N-[(3aR,6aS)-hexahydrocyclopenta[c]pyrrol-2(1H)-ylcarbamoyl]-4-methylbenzenesulfonamide 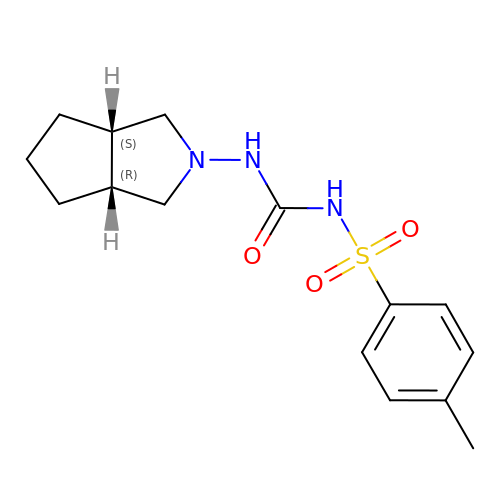| C15 H21 N3 O3 S | BOVGTQGAOIONJV-BETUJISGSA-N>ANSKEVKKRASSFEWFGSNESGAEFGSGNIPGVEGTDYTFPNTTAIQILIDAGMNIFRVPFLMERMIPTEMTGSLDTAYFEGYSEVINYITGKGAHAVVDPHNFGRYYGTPISSTSDFQTFWSTLASQFKSNDLVIFDTNNEYHDMDESVVVALNQAAIDGIRDAGATTQYIFVEGNAYSGAWTWTTYNTAMVNLTDPSDLIVYEMHQYLDSDGSGTSDQCVSSTVGQERVVDATTWLQSNGKLGILGEFAGGANSVCEEAVEGMLDYLAENSDVWLGASWWSAGPWWQDYIYSMEPPNGIAYESYLSILET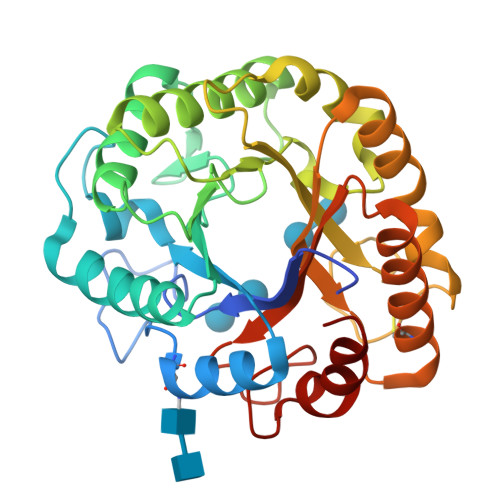YF[4x]> MHHHHHHHTGAAPDRKAPVRPTPLDRVIPAPASVDPGGAPYRITRGTHIRVDDSREARRVGDYLADLLRPATGYRLPVTAHGHGGIRLRLAGGPYGDEGYRLDSGPAGVTITARKAAGLFHGVQTLRQLLPPAVEKDSAQPGPWLVAGGTIEDTPRYAWRSAMLDVSRHFFGVDEVKRYIDRVARYKYNKLHLHLSDDQGWRIAIDSWPRLATYGGSTEVGGGPGGYYTKAEYKEIVRYAASRHLEVVPEIDMPGHTNAALASYA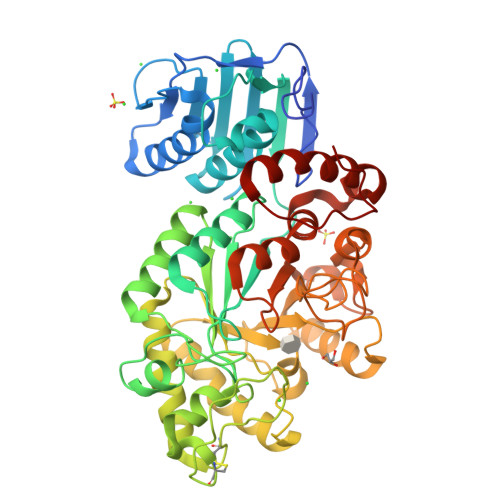ELNCDGVAPPLYTGTKVGFSSLCVDKDVTYDFVDDVIGELAALTPGRYLHIGGDEAHSTPKADFVAFMKRVQPIVAKYGKTVVGWHQLAGAEPVEGALVQYWGLDRTGDAEKAEVAEAARNGTGLILSPADRTYLDMKYTKDTPLGLSWAGYVEVQRSYDWDPAGYLPGAPADAVRGVEAPLWTETLSDPDQLDYMAFPRLPGVAELGWSPASTHDWDTYKVRLAAQAPYWEAAGIDFYRSPQVPWT> NCLPDWSVYEGYCYKVFKERMNWADAEKF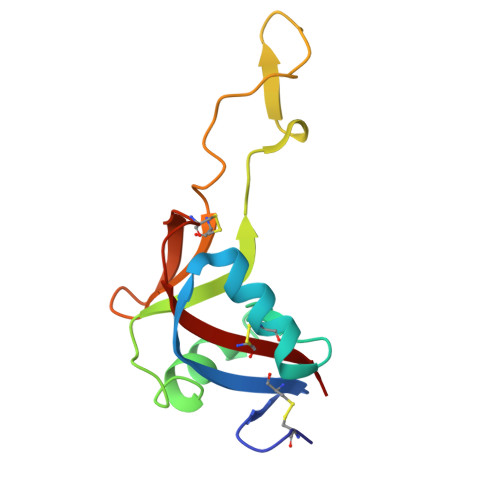CTKQHKDGHLVSFRNSKEVDFVISLAFPMLKNDLVWIGLTDYWRDCNWEWSDGAQLDYKAWDNERHCFIYKNTDNQWTRRDCTWTFSFVCKCPA>[2x]GHMATAPRPLREQYLHFQPISTRWHDNDIYGHVNNVTYYAFFDTAVNTYLIERGGLDIQGGEVIGLVVSSSCDYFAPVAFPQRIEMG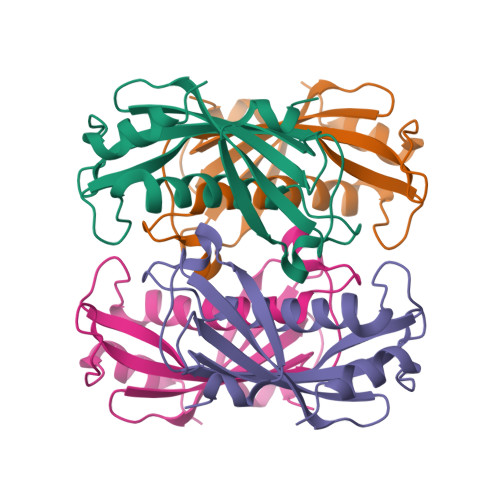LRVARLGNSSVQYELALFLEGQREACAAGRFVHVFVERRSSRPVAIPQELRDALAALQSSAQ>GQDMVSPPPPIADEPLTVNTGIYLIECYSLDDKAETFKVNAFLSLSWKDRRLAFDPVRSGVRVKTYEPEAIWIPEIRFVNVENARDADVVDISVSPDGTVQYLERFSARVLSPLDFRRYPFDSQTLHIYLIVRSVDTRNIVLAVDLEKVGKNDDVFLTGWDIESFTAVVKPANFALEDRLESKLDYQLRISRQYFSYIPNIILPMLFILFISWTAFWSTSYEANVTLVVSTLIAHIAFNILVETNLPKTPYMTYTGAIIFMIYLFYFVAVIEVTVQHYLKVESQPARAASITRASRIAFPVVFLLANIILAFLFFGF[5x]

GLIC is a bacterial homologue of the pentameric ligand-gated ion channels (pLGICs) that mediate the fast chemical neurotransmission of nerve signalling in eukaryotes. Because the activation and allosteric modulation features are conserved among prokaryotic and eukaryotic pLGICs, GLIC is commonly used as a model to study the allosteric transition and structural pharmacology of pLGICs. Unlike the other pLGICs, GLIC displays a particular activation mechanism in which protons, rather than a sizable agonist, trigger ion-channel opening. Here, experimental evidence for carboxylate binding to GLIC is provided by solving its X-ray structures with a series of monocarboxylate and dicarboxylate derivatives, and two carboxylate-binding sites are described: (i) the ‘intersubunit’ site that partially overlaps the canonical pLGIC orthosteric site and (ii) the ‘intrasubunit’ vestibular site, which is only occupied by a subset of the described derivatives.

Here, we solved a 3.2 Å resolution structure of GLIC in complex with propionate obtained from crystals grown in a solution buffered at pH 4.0 using 100 mM propionate instead of acetate. The overall structure was similar to the acetate-bound structure (root-mean-square deviation of below 0.3 Å calculated over 310 residues), and no significant remodelling of the intrasubunit and intersubunit pockets was observed upon propionate binding. Besides this sub-orthosteric intersubunit site, we show here that the intrasubunit site can accommodate some of the carboxylates described in this study, namely propionate and succinate. At the molecular level, all of the carboxylates bind to the intersubunit site that partially overlaps the pLGIC orthosteric site, but only acetate, propionate and succinate bind in the intrasubunit vestibular site.> MSSGPIFSSLVTDSSRSSRKKSDSALGTEFTVVCDRVPLRDPSPTVQRFLCFVFDNGSGAMSTLPIDVGGEGISLSDMKEVKAMPHIASGCTAVWGPPLPPKPGKDTKQVILWGGLDKRRWCCSNDLTQVDITITPKTTTAKVSILPADKQDGVPSPRTGHTLVAISSLQAILFGGLELASRHARLGTCAQSCKDGYFYLLDMTTLRWNKLPLPPLVPRAYHSSTWVPASSTMVIVGGITYSGHCPSERLSVSDVVCLKISDTSQYTLTEIHMEGVRDSYVSSSSASALCDDRFVLYGGYHHDKSGLHPPEPSRDLYVMNLQTKKAVVHHAPTRMASAGHTCLRLIDN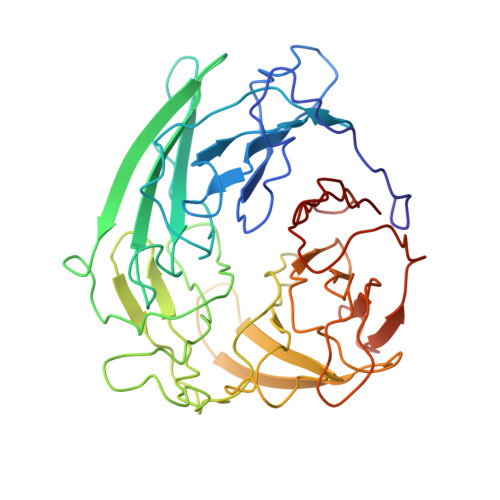SVVMIGGTCKSVNCCTNL> MSTAAKQNRSTSRVSKKKTAAPKEGAAKKSDKGHKYEYVELAKASLTSAQPQHFYAVVIDATFPYKTNQERYICSLKIVDPTLYLKQQKGAGDASDYATLVLYAKRFEDLPIIHRAGDIIRVHRATLRLYNGQRQFNANVFYSSSWALFSTDKRSVTQEINNQDAVSDTTPFSFSSKHATIEKNEISILQNLRKWANQYFSSYSV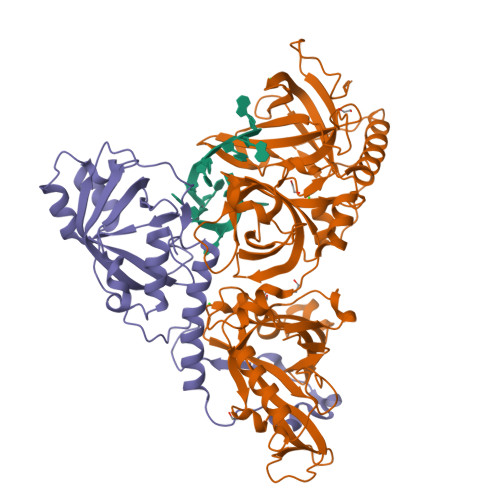ISSDMYTALNKAQAQKGDFDVVAKILQVHELDEYTNELKLKDASGQVFYTLSLKLKFPHVRTGEVVRIRSATYDETSTQKKVLILSHYSNIITFIQSSKLAKELRAKIQDDHSVEVASLKKNVSLNAVVLTEVDKKHAALPSTSLQDLFHHADSDKELQAQDTFRTQFYVTKIEPSDVKEWVKGYDRKTKKSSSLKGASGKGDNIFQVQFLVKDASTQLNNNTYRVLLYTQDGLGANFFNVKADNLHKNADARKKLEDSAELLTKFNSYVDAVVERRNGFYLIKDTKLIY;> MSKGASAPQQQSAFKQLYTELFNNEGDFSKVSSNLKKPLKCYVKESYPHFLVTDGYFFVAPYFTKEAVNEFHAKFPNVNIVDLTDKVIVINNWSLELRRVNSAEVFTSYANLEARLIVHSFKPNLQERLNPTRYPVNLFRDDEFKTTIQHFRHTALQAAINKTVKGDNLVDISKVADAAGKKGKVDAGIVKASASKGDEFSDFSFKEGNTATLKIADIFVQEKGKDALNKAADHTDGAKVKGGAKGKGKAAAKAAKGKKLSAKKGDSSAADVRKSVDKIVKYTPSKGSRKDTPQKSQAPAAGKSSAKKGGKKAVPSAPSPSGKKSALTTDKMTMAQFVKYLDWHEKKKGGKVSSGGKVLGKRSAGKASATSGKASKASKKTAAKK1-[[(4-PHENOXYPHENYL)SULFONYL]AMINO]-3-[[N/N-(4-PYRIDINYLCARBONYL)-L-LEUCYL]AMINO]-2-PROPANOL | C27 H32 N4 O6 S | 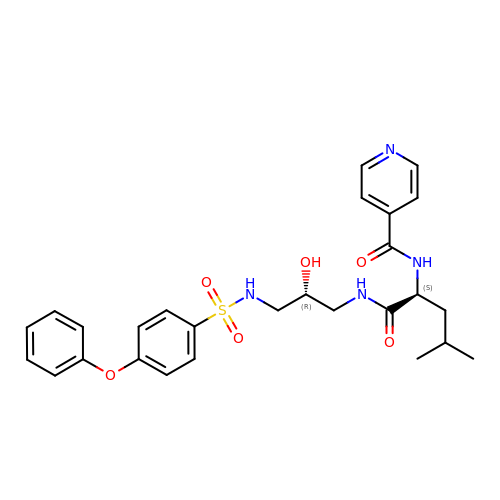RNXGMLBGKGGGPZ-BWKNWUBXSA-N Cys-loop receptors are a class of pentameric ligand-gated ion channels that are activated by specific neurotransmitters, including acetylcholine (ACh), serotonin (5-HT), glycine (Gly), and γ-aminobutyric acid (GABA). Recently, Gao et al. characterized an extensive set of mutants in acetylcholine binding protein (AChBP), a structural and functional homolog of the extracellular domain of the nAChR. Using X-ray crystallography we solved 3-dimensional structures of strychnine or d-tubocurarine in complex with ACh binding protein (AChBP), a well-recognized structural homolog of the nicotinic ACh receptor. Our results demonstrate that AChBP binds strychnine and d-TC with high affinity and serves as an appropriate model for mapping the binding site topography in different CLRs, including the GlyR, nAChR, and 5-HT3R.

Similarly, we found that the affinity of d-TC for Ac-AChBP (Ki = 509.2±38.0 nM) is in the same range as the reported values for binding of d-TC at muscle nAChR and the mouse 5-HT3R. The asymmetric unit contains two pentamers, which interact through loop C and form an interface that resembles the one seen in the strychnine complex. Inspection of simple difference electron density revealed occupancy of most of the binding sites by d-TC. Remarkably, at least three different binding orientations of d-TC can be distinguished (indicated with binding mode 1–3). Binding mode 1 (yellow) occurs at most binding sites, but with ligand occupancies that vary between 30% and 60%. d-TC molecules were not built in binding sites if the electron density indicated partial occupancy. In binding mode 1, the tertiary amine group of d-TC forms a hydrogen bond with the carbonyl oxygen of W145 and forms cation-π interactions with conserved aromatic residues of the binding pocket. A second ligand orientation (mode 2, magenta) occurs only once in the pentamer and is characterized by a polar interaction between the quaternary amine group of d-TC and the carbonyl oxygen of W145. A superposition of the (+) face in binding mode 1 (protein shown in yellow) and the (+) face in binding mode 2 (protein and ligand shown in magenta) shows that the different ligand orientation in mode 2 results in an outward displacement of the tip of loop C by a distance of 4.5 Å relative to mode 1. Finally, difference electron density at one of the binding sites involved in a crystal contact between neighboring C loops indicates the occupancy by a single ligand likely adopting multiple binding orientations. Consequently, these different ligand binding modes result in varying conformations of loop C and stabilize the homopentameric AChBP in a structurally asymmetric state.

>QANLMRLKSDLFNRSPMYPGPTKDDPLTVTLGFTLQDIVKVDSSTNEVDLVYYEQQRWKLNSLMWDPNEYGNITDFRTSAADIWTPDITAYSSTRPVQVLSPQIAVVTHDGSVMFIPAQRLSFMCDPTGVDSEEGVTCAVKFGSWVYSGFEIDLKTDTDQVDLSSYYASSKYEILSATQTRQVQHYSCCPEPYIDVNLVVKFRERRAGNGFFRNLFD[10x]> HHHHHHMQAQVFRVPMSNPADVSGVAKLIDEGVIRAEEVVCVLGKTEGNGCVNDFTRGYTTLAFKVYFSEKLGVSRQEVGERIAFIMSGGTEGVMAPHCTIFTVQKTDNKQKTAAEGKRLAVQQIFTREFLPEEIGRMPQVTETADAVRRAMREAGIADASDVHFVQVKCPLLTAGRMHDAVERGHTVATEDTYESMGYSRGASALGIALALGEVEKANLSDEVITADYSLYSSVASTSAGIELMNNEIIVMGNSRAWGGDLVIGHAEMKDAIDGAAVRQALRDVGC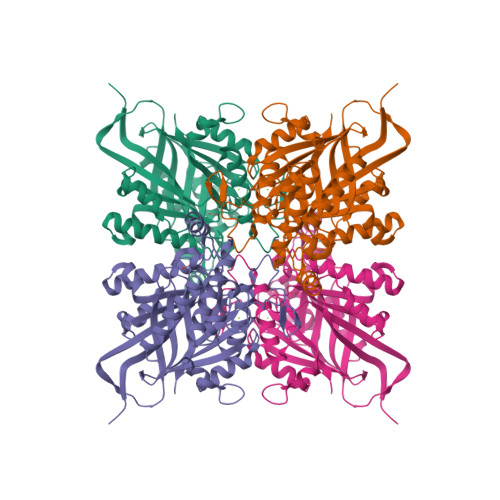CENDLPTVDELGRVVNVFAKAEASPDGEVRNRRHTMLDDSDINSTRHARAVVNAVIASIVGDPMVYVSGGSEHQGPAGGGPVAVIARTA>MRAVRLVEIGKPLSLQEIGVPKPKGPQVLIKVEAAGVCHSDVHMRQGRFGNLRIVEDLGVKLPVTLGHEIAGKIEEVGDEVVGYSKGDLVAVNPWQGEGNCYYCRIGEEHLCDSPRWLGINFDGAYAEYVIVPHYKYMYKLRRLNAVEAAPLTCSGITTYRAVRKASLDPTKTLL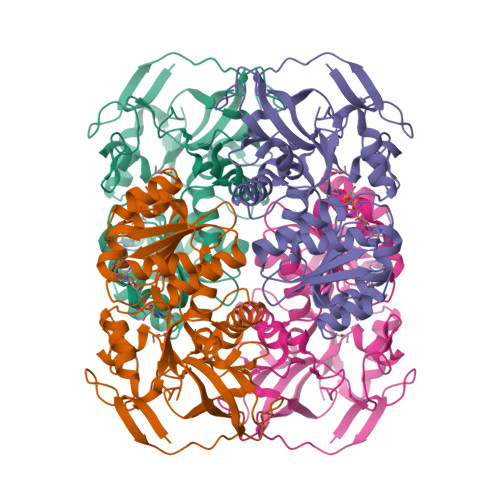VVGAGGGLGTMAVQIAKAVSGATIIGVDVREEAVEAAKRAGADYVINASMQDPLAEIRRITESKGVDAVIDLNNSEKTLSVYPKALAKQGKYVMVGLFGADLHYHAPLITLSEIQFVGSLVGNQSDFLGIMRLAEAGKVKPMITKTMKLEEANEAIDNLENFKAIGRQVLIP[2x]>MKDLSHYGPALCVKFYNDYVLAGYGPFIHVYDYHSATLINKCRLFHYNKVHGLSLSSEGKILAYGARSVTIVELEDVLKKESLVDFERINSDWITGATFSFDNLQIYLLTCYNKVLICDLNCEVLFRKSLGGERSILYSGIIKVFGPDKVYVNAGTVMGGVIIWDLFSETKIHNLLGHEGSIFYVNLSNNGRYVASCSDDRSIRLWDLETGKQLSVGWSHTARIWNLMFFDNDSKLISVSEDCTCRVWNIIESRENVAELSISNVYEVHLIKSIWGVDVKDDEMIAVTSGNDGRLKLIDLLQLKRHGDEETSFSLDDIAKQCGDIFEKNESIKGFQWFSFGVIAITSLGKILKYSDVTKQWKLLLTNEKFNSYPITNGIQTQNIAVFSNNKSDILLIKFSKDSADIIETEEFHLDELSKTNNCLVTEYDDDSFLLTLQSPNPREKFVCLEISLQNLKIKSKHCFNKPENFSSSCLTSFRNHILVGSRFSTLVIYNLLDESEEPFIIRRLSPGDTTTSIEFVEDKDNSAVFSVTNRDGYYVFIELTKNSLEEGPYRLSYKVLHSNKMMKGFLEGAFFNSKGEYITYGFKSSLFYLYNETNCYELASEVCGGSHRLWNLAKITDGHVLMYIKASRFHLRKIYNSIVPETLENGVHGREIRDISICPVSNTNTNDNFKDGHIFCTASEDTTIKLGYFNNRTGKVQNFWTQRKHVSGLQRCQFINHKLMISSSAREELFLWELNDKYNKRPYMTIRQALPVSTNNSDLRIMDFDVKFISQSGDFLLVTVYSDSTIKIWHYRENQNKFDLIMQGRYKTCCLFNVVFIALKEELLVVISPTDGHLVVYNITEYVPFSVDPISGDLVDHKLDATISNLPAPVAQLPVHQSGVKSLDYVANATRTSATILTGGDDNGLGLSNLKLDDSNKVTLKTSDFIAAAASSTITSGMLINGGKEVITTSVDQVIRAWEITAGKLSLVDKKRTTVADTGSLEIISNDEDADSEKTLLIGGVGLSIWKKLEVLFQGPSHHHHHH[2x];>[2x]MGKSSKDKRDLYYRKAKEQGYRARSAFKLLQLNDQFHFLDDPNLKRVVDLCAAPGSWSQVLSRKLFDESPSSDKEDRKIVSVDLQPMSPIPHVTTLQADITHPKTLARILKLFGNEKADFVCSDGAPDVTGLHDLDEYVQQQLIMSALQLTACILKKGGTFVAKIFRGRDIDMLYSQLGYLFDKIVCAKPRSSRGTSLEAFIVCLGYNPPSNWTPKLDVNTSVDEFFQGCFLNKLCISDKLSHWNEEERNIAEFMACGSLQSFDSDATYHDLPSSVAGTS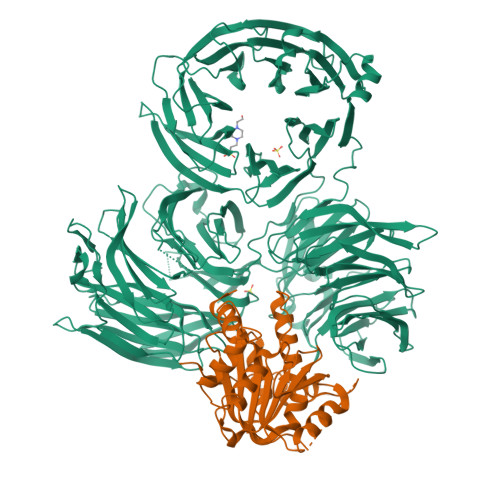SSLDPVQSPTNPPYKKALELKRSGKLTRSVLEVLFQGPSHHHHHH> ADEIGDAAKKLGDASYAFAKEVDWNNGIFLQAPGKLQPLEALKAIDKMIVMGAAADPKLLKAAAEAHHKAIGSVSGPNGVTSRADWDSVLAALGRVIASVP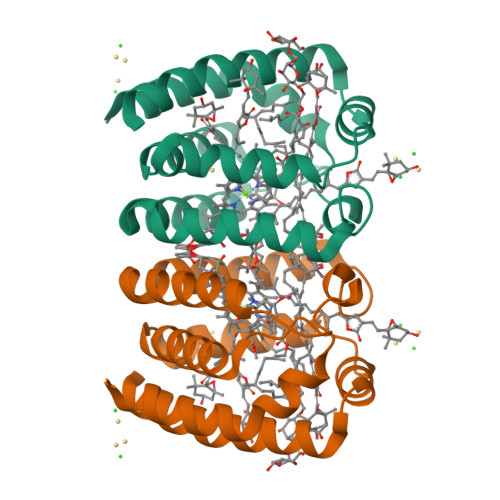ENMVMDVYDSVSKITDPKVPAYMKSLVNGADAEKAYEGFLAFKDVVKKSQ> DIEQLSFARGLAIDETNDHQYKLTYQNLLPQSEDSQASGKPEFVNVTSHGKTILEAVSDVSIKDPPVYSDHLKVILLGEKLMRNQNVDQVLNHFIRDDELRRSSYLMAARGNAADVFTKGNPNQQQPMPSEKLIDLTTHSGYNGKIMIPLRIGRASVYSQNGYSYLIQAVKNEKGKAKYDGAGIIKRGSNKLVGFLSADETQTLSWVMGTIQGGVMPTTDKGHPITFEIKKSKTKIKPVIENGKP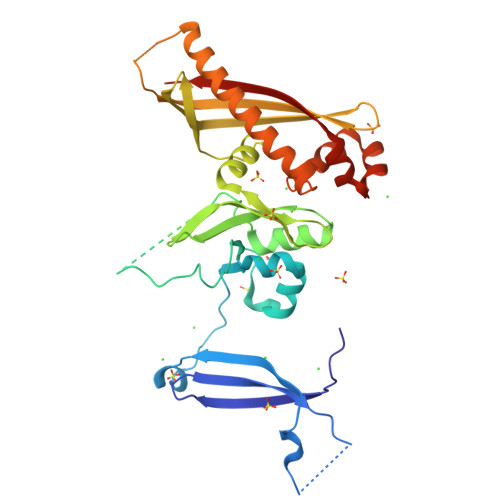VFHISVKTKGILTEDQNPNENSFSKSYLHRLENIFEKKLERDVKQVMDKLQHEYKTDPVFLSDHIRIQHPDYWNKVKGHWDEIFSETDFKYDISFKIINFGTVGK>MGSKAILLFDVDGTLTPPRNPETHDMKEALLKARAAGFKLGVVGGSDFAKQKEQLGESILEDFDYVFSENGLLAYKDGKEFHRNSLLRALGNEKVVAFVKKCLHLIADLDIPVQRGTFVEFRNGMFNVSPIGRNCSQQERDEFENLDKERHIREKLIR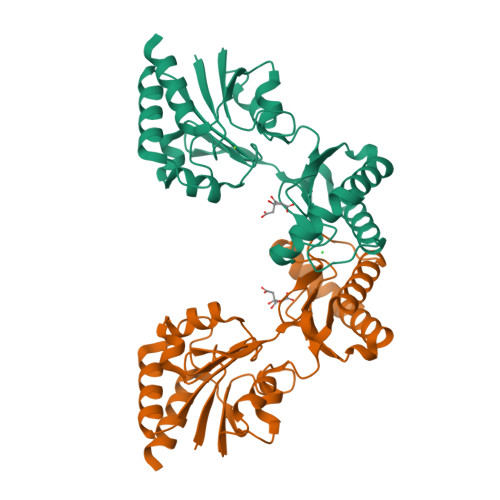ELKEAFPDYQLAYSVGGQISFDVFPKGWDKTYCLQFVENDFETIHFFGDKTSEGGNDYEIFTDSRTIGHSVKTYKDTIAILEALLEDSR[3x]> ETGSERCDDWGLDTMRQIQVFEDEPARIKCPLFEHFLKYNYSTAHSSGLTLIWYWTRQDRDLEEPINFRLPENRISKEKDVLWFRPTLLQDTGQYTCMLRNTTYCSKVAFPLEVVQKDSCFNSAMRFPVHKMYIEHGIHKITCPNVDGYFPSSVKPSVTWYKGCTEIVDFHNVLPEGMQLSFFIPLVSNNGQYTCVVTYPENGRLFHLTRTVTVKVVGSPKDALPPQIYSPNDRVVYEKEP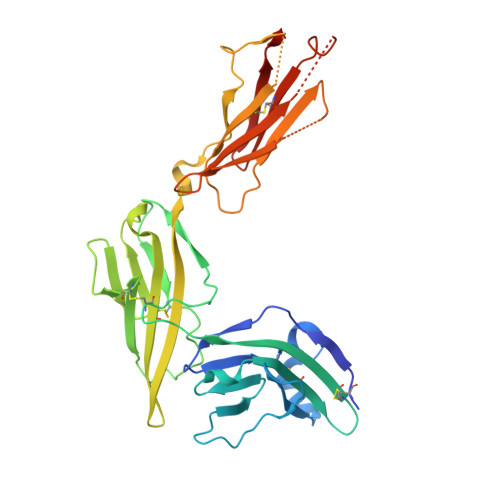GEELVIPCKVYFSFIMDSHNEVWWTIDGKKPDDVTVDITINESVSYSSTEDETRTQILSIKKVTPEDLRRNYVCHARNTKGEAEQAAKVKQKHHHHHH>KTNTATVKVLPISMSDEGDSFLVKDSLGENKIPKNPSKVVILDLGILDTFDALKLNDKVVGVPAKNLPKYLQQFKNKPSVGGVQQVDFEAINALKPDLIIISGRQSKFYDKLKEIAPTLFVGLDNANFLSSFENNVLSVAKLYGLEKEALEKISDIKNEIEKAKSIVDEDKKALIILTN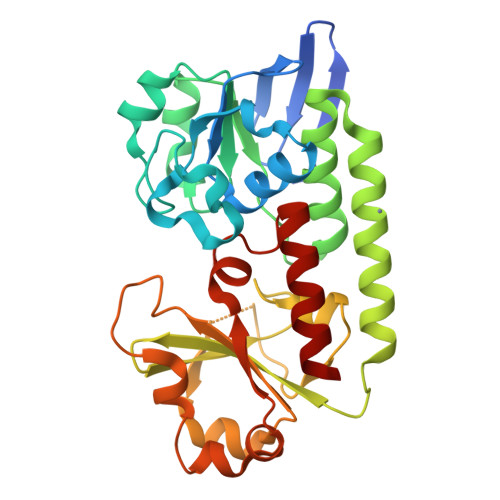SNKISAFGPQSRFGIIHDVLGINAVDENIKVGTHGKSINSEFILEKNPDYIFVVDRNVILGNKERAQGILDNALVAKTKAAQNKKIIYLDPEYWYLASGNGLESLKTMILEIKNAVK[2x]> MSEPIDILIAGAGIGGLSCALALHQAGIGKVTLLESSSEIRPLGVGINIQPAAVEALAELGLGPALAATAIPTHELRYIDQSGATVWSEPRGVEAGNAYPQYSIHRGELQMILLAAVRERLGQQAVRTGLGVERIEERDGRVLIGARDGHGKPQALGADVLVGADGIHSAVRAHLHPDQRPLSHGGITMWRGVTEFDRFLDGKTMIVANDEHWSRLVAYPISARHAAEGKSLVNWVCMVPSAAVGQLDNEADWNRDGRLEDVLPFFADWDLGWFDIRDLLTRNQLILQYPMVDRDPLPHWGRGRITLLGDAAHLMYPMGANGASQAILDGIELAAALARNADVAAALREYEEARR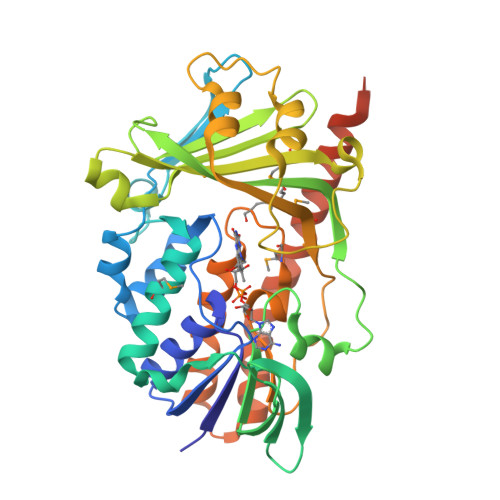PTANKIILANREREKEEWAAASRPKTEKSAALEAITGSYRNQVERPR>[2x]MKVGQDKVVTIRYTLQVEGEVLDQGELSYLHGHRNLIPGLEEALEGREEGEAFQAHVPAEKAYGATGHPGIIPPHATLDFQVEVVK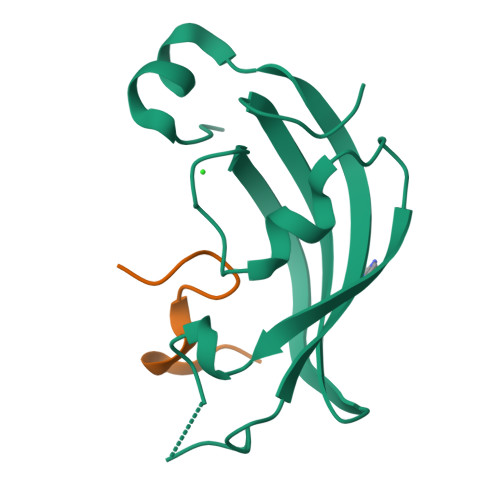VREATPEELLHGHAHPSGHHHHHH;>TRYWNAKALPFAFGA[2x]(4R,5S,6S)-6-((R)-1-hydroxyethyl)-3-((2-isopropoxy-2-oxoethyl)thio)-4-methyl-7-oxo-1-azabicyclo[3.2.0]hept-2-ene-2-carboxylic 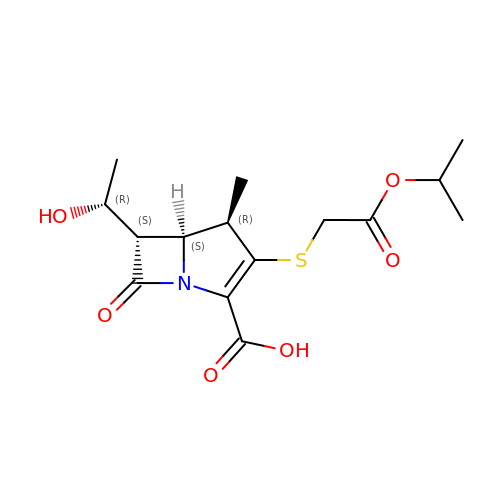acid | C15 H21 N O6 S | ZNVHAIJDJMRLJY-YJFSRANCSA-N> ANIVGGIEYSINNASLCSVGFSVTRGATKGFVTAGHCGTVNATARIGGAVVGTFAARVFPGNDRAWVSLTSAQTLLPRVANGSSFVTVRGSTEAAVGAAVCRSGRTTGYQCGTITAKNVTANYAEGAVRGLTQGNACMGRGDSGGSWITSAGQAQGVA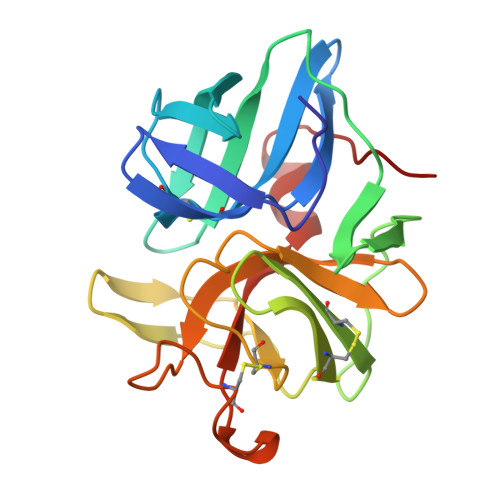SGGNVQSNGNNCGIPASQRSSLFERLQPILSQYGLSLVTG>MGGSHHHHHHGMASHKLLVTPPKALLKPLSIPNQLLLGPGPSNLPPRIMAAGGLQMIGSMSKDMYQIMDEIKEGIQYVFQTRNPLTLVISGSGHCALEAALVNVLEPGDSFLVGANGIWGQRAVDIGERIGARVHPMTKDPGGHYTLQEVEEGLAQHKPVLLFLTHGESSTGVLQPLDGFGELCHRYKCLLLVNSVASLGGTPLYMDRQGIDILYSGSQKALNAPPGTSLISFSDKAKKKMYSRKTKPFSFYLDIKWLANFWGCDDQPRMYHHTIPVISLYSLRESLALIAEQGLENSWRQHREAAAYLHGRLQALGLQLFVKDPALRLPTVTTVAVPAGYDWRDIVSYVIDHFDIEIMGGLGPSTGKVLRIGLLGCNATRENVDRVTEALRAALQHCPKKKL[8x]

AGT is a hepatocyte-specific PLP dependent enzyme, belonging to the Fold Type I family, catalysing the transamination reaction between L-alanine and glyoxylate to produce glycine and pyruvate, thus leading to the removal of glyoxylate. AGT normally localises in the peroxisomes and failure of its detoxification role leads to increased levels of oxalate, coming from oxidation of glyoxylate, causing calcium oxalate precipitation in the kidney and urinary tract. Many pathogenic variants of AGT cause PH1 (primary hyperoxaluria type I), a rare autosomal recessive disorder. Our results shows that two forces generated by the salt bridge between the conserved aspartate residue and the pyridine N1 atom, and by the Schiff base linkage act as opposite springs and are responsible for the fine tilting adjustments of the pyridine plane of PLP.

D183N is a pathogenic variant of AGT that causes Primary Hyperoxaluria Type I (PH1), a severe disorder of glyoxylate metabolism. Although the mutation is conservative, the variant shows a 2.3 × 104 fold reduction of the catalytic efficiency, whereas the affinity for PLP is almost unchanged. Following our novel hypothesis, and to understand if the low catalytic efficiency may be due to a non-native geometrical strain, we have solved the structure of the D183N mutant at 1.8 Å resolution and at a similar pH value (pH 5.5 vs 5.0) of the wild type. The structure of D183N shows that the interaction of the asparagine side chain with N1 is loosen, going from a 2.6 Å distance in the wild type to 3.0 Å. As a consequence of the strain relaxation, the torsion angle between the imine and pyridine planes is reduced by 10° (from 36.2° to 26.3°) and the cofactor tilts in the direction of the Lys (si face), assuming a conformation that superposes very well with the geometrically optimized reduced internal aldimine. Clearly, the H-bond between the mutated Asn amino group and the deprotonated pyridine N1 is not as strong as the salt bridge present in the wild type enzyme. Therefore, in the mutant the opposite torsion effect is uncoupled and the spring mechanism, responsible for the tilt of the PLP pyridine plane during the transaldimination step, is lost. In the D183N variant the H-bond replacing the salt bridge isn’t strong enough to keep the internal aldimine under strain and the pyridine plane is tilted towards the si side, whereas in the S187F variant the salt bridge is conserved but the counter pulling force of the Schiff base linkage is lost, due to the rearrangement of the Lys-209 loop, and the pyridine plane of the internal aldimine is tilted towards the re side.>MDIWYGTAAVPKDLDNSAVTIGVFDGVHRGHQKLINATVEKAREVGAKAIMVTFDPHPVSVFLPRRAPLGITTLAERFALAESFGIDGVLVIDFTRELSGTSPEKYVEFLLEDTLHASHVVVGANFTFGENAAGTADSLRQICQSRLTVDVIDLLDDEGVRISSTTVREFLSEGDVARANWALGRHFYVTGPVVRGAGRGGKELGWPTANQYFHDTVALPADGVYAGWLTILPTEAPVSGNMEPEVAYAAAISVGTNPTFGDEQRSVESFVLDRDADLYGHDVKVEFVDHVRAMEKFDSVEQLLEVMAKDVQKTRTLLAQDVQAHKMAPETYFLQAES[2x]

The FAD synthetase from Corynebacterium ammoniagenes (CaFADS) is a bifunctional enzyme responsible for the synthesis of flavin mononucleotide (FMN) and flavin adenine dinucleotide (FAD) cofactors. The C-terminal module catalyzes FMN synthesis from riboflavin (RF) (riboflavin kinase, RFK), while the N-terminal one transforms FMN into FAD (FMN:adenylyltransferase, FMNAT). Bioinformatic tools for the exploration of macromolecular interfaces predict that CaFADS might stabilize in hexameric assemblies in solution, organized as dimer of trimers. In the predicted CaFADS dimer of trimers model, the protomers adopt a head-to-tail organization within each trimer that causes the RFK and FMNAT catalytic sites of two neighboring protomers 6 to be in proximity.

The overall structures of F206W, D298E and E301A CaFADSs are quite similar to that of the WT (A chains r.m.s.d. values 0.149, 0.152 and 0.251 Å, superimposing 274, 309 and 317 atoms, respectively). Thus, in the F206W structure, residues 200–204 in chain A and 201–202 in chain B from L1c, as well as residues 259–263 (in chain A) and 261–264 (in chain B) from L4c-FlapII, are not observed. For the F206W variant, the side chain of the introduced tryptophan was refined in slightly different conformations for each of the two molecules of the asymmetric unit. Both differ from those of F206 in the WT structure and in the substrate-bound complex. Moreover, residues 197–199 on L1c-FlapI of F206W CaFADS were displaced relative to those of the WT, contributing to the opening of the cavity where ADP binds in the RFK module. Noticeably, these residues immediately precede the region that stabilizes a 310 α-helix (199–204) in the ternary complex structure of the CaFADS RFK module that contains the reaction products, FMN:ADP:Mg2+. The PISA server predicts a dimer of trimers for the F206W structure, in which the orientations of F62 and W206 side chains from the two neighboring protomers differ from the WT, and the distance between the aromatic rings increases by 1.34 Å. In the WT CaFADS dimer of trimers, K202 and E203 stabilize salt-bridges with E130 and N131 from loop L8n of the neighboring protomer within the trimer, while F206 interacts with F62 of helix α2n. The mutation of K202 and E203 to Ala would prevent formation of the salt-bridges, while substitution of F206 by Ala or Lys will abrogate its hydrophobic interaction with F62. With the elimination of such interactions, the shape of the isoalloxazine hydrophobic cavity in the FMNAT site should change, as found when evaluating this cavity in the dimer of trimers assembly for the F206W variant. This conservative substitution apparently reduces the amount of oligomeric assemblies able to bind FMN and FAD at the FMNAT site, relative to the WT, an effect that is clearly overcome in the ternary complex.>[2x]MVLYFIGLGLYDERDITVKGLEIAKKCDYVFAEFYTSLMAGTTLGRIQKLIGKEIRVLSREDVELNFENIVLPLAKENDVAFLTP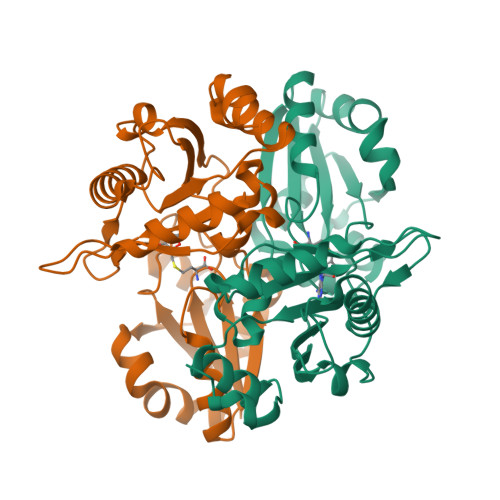GDPLVATTHAELRIRAKRAGVESYVIHAPSIYSAVGITGLHIMKFGKSATVAYPEGNWFPTSYYDVIKENAERGLHTLLFLDIKAEKRMYMTANEAMELLLKVEDMKKGGVFTDDTLVVVLARAGSLNPTIRAGYVKDLIREDFGDPPHILIVPGKLHIVEAEYLVEIAGAPREILRVNV> MAHHHHHHMNIDLTGRLALVTGASRGIGYFLSLELAKRGAHVIAVARTVGGLEELDDEIRKLGSSATLVPLDITDMEALDRLGGTIHERWGKLDILVANAGILGTISPIGHVEAKTFEKVMNINVTSVWRLIRSVDPLLRASDAGRAIMLSSGVAHSCRAF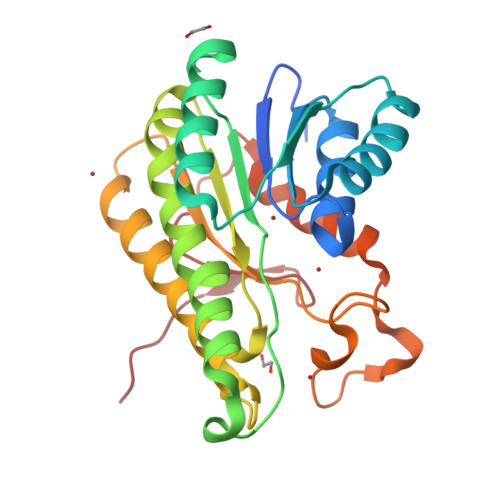WGPYAASKAAVEVMARCWAEETKKMKLKINSVNPGATRTAMRAQAMPGEDPETLPTPQSVAEKIVKLADPKLEVTGKLFDVRQDRFLDYHMPS3-methyl-1-(2-piperazin-1-yl-1,3-thiazol-4-yl)-2,5,6,7-tetrahydroisoindol-4-one 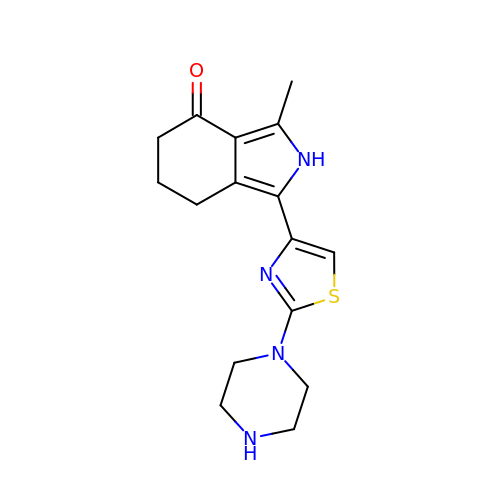| C16 H20 N4 O S | HRDOIKMHSZXEOA-UHFFFAOYSA-N> IDFVYRVDPNPPDVIFRDGFSLLGYNRDLQQLISGRSCAGGSSDSRYIVTTSDINKTYA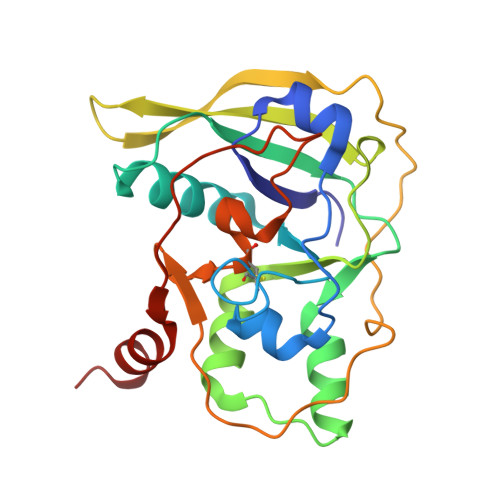IARAYYSHSKFKGNLYRYKIRADNNFYSLTPSVNYLESQGGHFNAYEKSMIRLQSEYVSTLSILPENIQKAVALVYDSSTGQIKDGTSTINTDYVSISSVSNPGVIPFLPEPQANTQQRIDAFGSLISSCFSIYSVCQTHRGQKTEVYKMPFYDARPVIQFIISGN> GS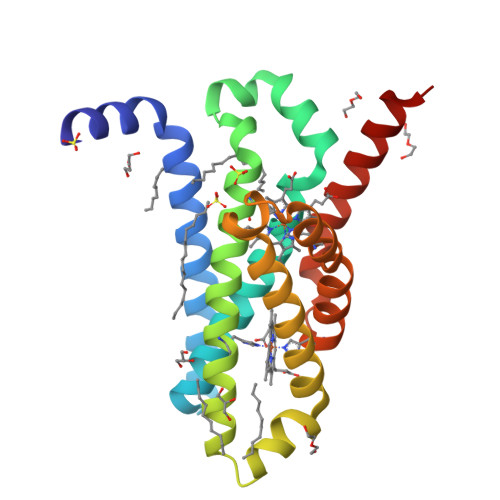AYIKYYIENNWVKIAFLALYVFVNMFFFMSAVEKYESQGANLYVQIARGCGATLNLNGALILIPMLRHFMTWLRKTTINNYIPIDESIEFHKLVGQVMFALAIVHTGAHFLNYTTLPIPFAQSLFGTKAGISGFLLLLVFIIMWVTAQAPIRKGGKFALFYIAHMGYVLWFALALIHGPVFWQWVLLPVVGFIIELVIRWKAAE>[6x]GGUCACAAC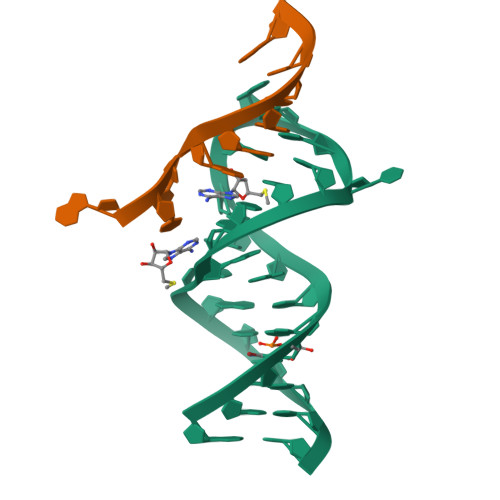GGCUUCCUGGCGUGACC;>AUUGGAGCA[6x]> CTMIPQYEQPKVEVAETFQNDTSVSSIRAVDLGWHDYFADPRLQKLIDIALERNTSLRTAVLNSEIYRKQYMIERNNLLPTLAANANGSRQGSLSGGNVSSSYNVGLGAASYELDLFGRVRSSSEAALQGYFASVANRDAAHLSLIATVAKAYFNERYAEEAMSLAQRVLKTREETYNAVRIAVQGRRDFRRRPAPAEALIESAKADYAHAARSREQARNALATLINRPIPEDLPAGLPLDKQFFVEKLPAGLSSEVLLDRPDIRAAEHALKQANANIGAARAAFFPSIRLTGSVGTGSVELGGLFK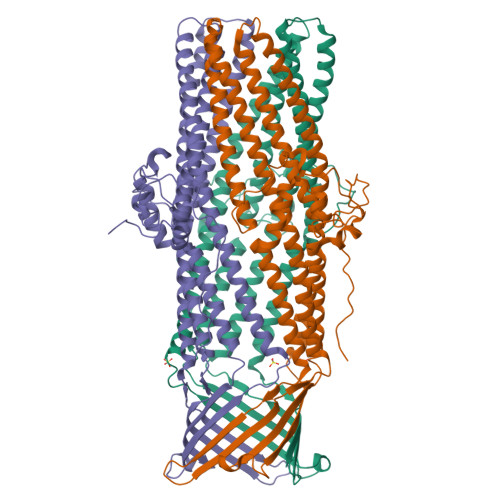SGTGVWAFAPSITLPIFTWGTNKANLDVAKLRQQAQIVAYESAVQSAFQDVANALAAREQLDKAYDALSKQSRASKEALRLVGLRYKHGVSGALDLLDAERSSYSAEGAALSAQLTRAENLADLYKALGGGLKRDTQTGK> PSIGLVIDKKEKVIDAK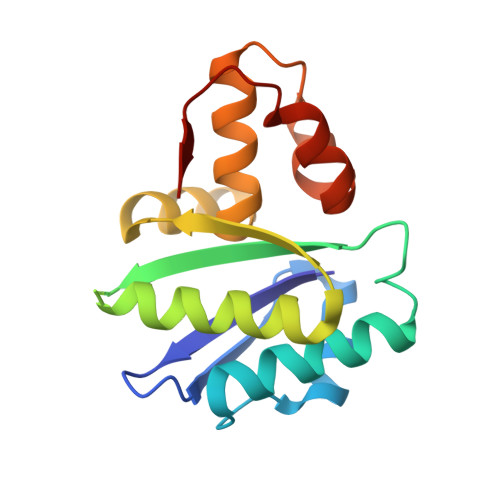PLNNDAKPILDEAAPKDMPLYDALSKILDISKKNGYINSADNIVLFSASINSGRNNVSESDKGIQEIISTLKDVAKDAGVKFEIIPSTEEDRQKALDQNLSMGRYAIYVKAVEEGVNLNLEDARNLSVSEILGKVNIGKFAISDT> MSPAPVQVMGVLNVTDDSFSDGGCYLDLDDAVKHGLAMAAAGAGIVDVGGESSRPGATRVDPAVETSRVIPVVKELAAQGITVSIDTMRADVARAALQNGAQMVNDVSGGRADPAMGPLLAEADVPWVLMHWRAVSADTPHV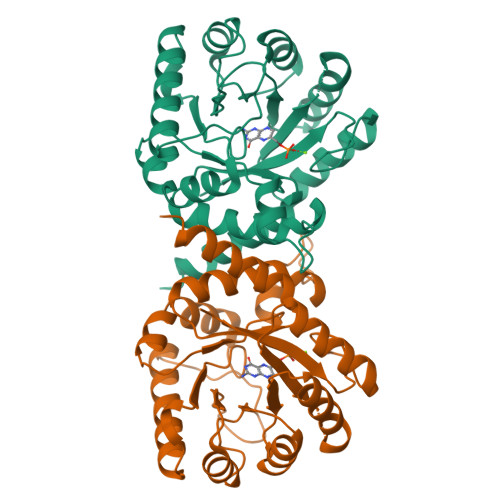PVRYGNVVAEVRADLLASVADAVAAGVDPARLVLDPGLGFAKTAQHNWAILHALPELVATGIPVLVGASRKRFLGALLAGPDGVMRPTDGRDTATAVISALAALHGAWGVRVHDVRASVDAIKVVEAWMGAERIERDG>MTETTENVVITIPDKTSFTFHEAATSPSEGEEFVVGHFRELTVKISGSSTSREIKFYAVDENGEKTALSGTNKTDFQLGSSTLNTNEYWDFDIAGLFKVMFEVVSVTGDVTVKGIVVS[5x]

In order to elucidate their role in the lytic cassette of B. subtilis prophages, we cloned and produced XepA from the PBSX prophage and YomS from the SPβ prophage. The putative lysins XepA and YomS align very well, with a sequence identity of 38% (54% similarity) covering 85% of the overall sequence. The C-terminal disc of XepA is very similar to the structure of YomS, and the full-length protein including both domains is essential for cytotoxic activity. Both the XepA and YomS monomeric β-sandwiches adopt a fold resembling the C2 domain, which usually contains about 110 amino acids and 2–3 Ca2+ ions. In summary, we show that XepA initiates cell death in vivo, whereas YomS has no effect.

However, YomS corresponds to the C-terminal half of XepA. The three-dimensional structure of YomS was determined to a resolution of 1.3 Å by SeMet SAD phasing. YomS adopts an antiparallel β-sandwich fold, which arranges as a pentameric disc similar to the C-terminal domain of XepA. In this disc the monomers can be superimposed on each other with an r.m.s.d. of 0.1–0.2 Å. Comparing YomS with the C-terminal domain of XepA shows that the structures are highly conserved, as presented in Fig. 7. The individual interfaces within the pentamers of both proteins show extensive electrostatic interactions. The buried surfaces between two XepA chains and two YomS chains amount to approximately 3300 and 1100 Å2, respectively. Rather than being based on one or two key residues, the interfaces are mainly held together by a large number of hydrogen bonds (over 40 for XepA and approximately 20 for YomS) and salt bridges. YomS does not exhibit any effects on the tested bacteria. However, the XepA C-terminal domain and YomS may bind to the capsid in a vertex position according to their fivefold symmetry, stabilizing the virus particle (YomS) and helping the virus particle to escape (XepA).> MGSDKIHHHHHHMYTREELMEIVSERVKKCTACPLHLNRTNVVVGEGNLDTRIVFVGEGPGEEEDKTGRPFVGRAGMLLTELLRESGIRREDVYICNVVKCRPPNNRTPTPEE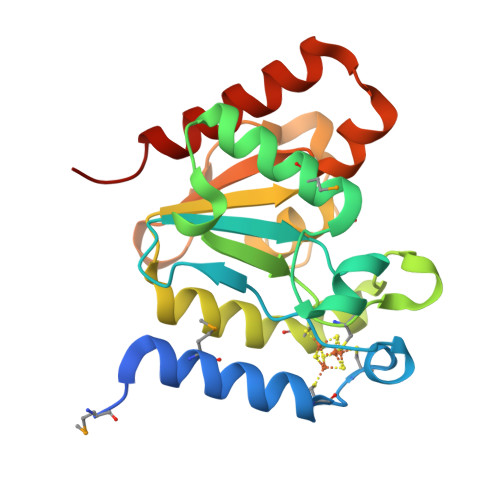QAACGHFLLAQIEIINPDVIVALGATALSFFVDGKKVSITKVRGNPIDWLGGKKVIPTFHPSYLLRNRSNELRRIVLEDIEKAKSFIKKEG>[2x]MTSQEKSMPFIKHLASSDRKVRTAALNSLHAFLSARQVASALTTLDVLKLWKGLFYALWMCDRAIPQQNLCNELADLIWQLPRESVATWLRGFWATMAREWTGIDVLRMEKFLLLVRRVLGASFKWMKKDGSLGKRTHDGQEKAVKTGAWDQSKVDEVLGLLAEWPFSLAEEVRITQSSEKGGEIVQKIPVGMRLHVLDIWVDEVE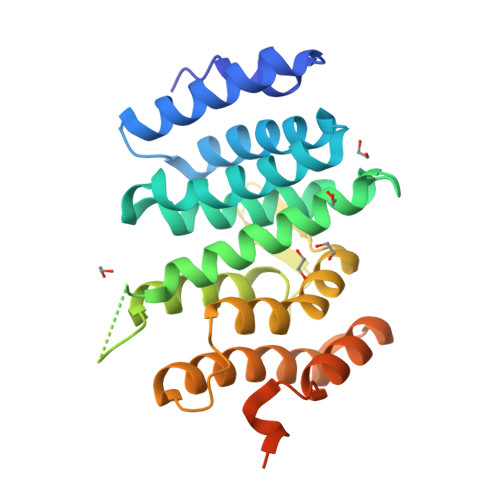RVGLLNEDEEEARMIVQRISDMVDALEQTTKSPAVRTRSKDSLGDDRLPANRRPNSSQDHDTKDMGDSDSWEGFDDGSHHHHHH>[4x]MPVDKNLRDLEPGIHTDLEGRLTYGGYLRLDQLLSAQQPLSEPAHHDEMLFIIQHQTSELWLKLLAHELRAAIVHLQRDEVWQCRKVLARSKQVLRQLTEQWSVLETLTPSEYMGFRDVLGPSSGFQSLQYRYIEFLLGNKNPQML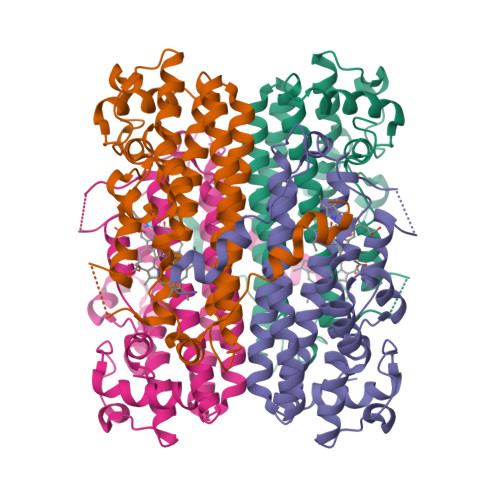QVFAYDPAGQARLREVLEAPSLYEEFLRYLARFGHAIPQQYQARDWTAAHVADDTLRPVFERIYENTDRYWREYSLCEDLVDVETQFQLWRFRHMRTVMRVIGFKRGTGGSSGVGFLQQALALTFFPELFDVRTSVGVDNRPPQGSADAGKRLEHHHHHH>XMKQYLELMQKVLDEGTQKNDRTGTGTLSIFGHQMRFNLQDGFPLVTTKRCHLRSIIHELLWFLQGDTNIAYLHENNVTIWDEWADENGDLGPVYGKQWRAWPTPDGRHIDQITTVLNQLKNDPDSRRIIVS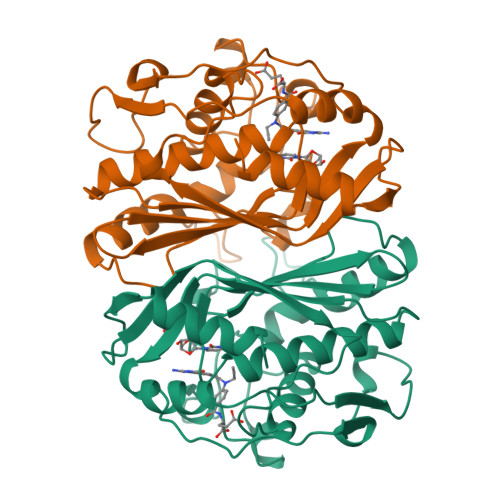AWNVGELDKMALAPCHAFFQFYVADGKLSCQLYQRSCDVFLGLPFNIASYALLVHMMAQQCDLEVGDFVWTGGDTHLYSNHMDQTHLQLSREPRPLPKLIIKRKPESIFDYRFEDFEIEGYDPHPGIKAPVAI[2x]>MGHHHHHHHHHHMSKQQIGVVGMAVMGRNLALNIESRGYTVSVFNRSREKTEEVIAENPGKKLVPYYTVQEFVESLETPRRILLMVKAGAGTDSAIDSLKPYLDKGDIIIDGGNTFFQDTIRRNRELSAEGFNFIGTGVSGGEEGTLKGPSIMPGGQKEAYELVAPILKQIAAVAEDGEPCVTYIGADGAGHYVKMVHNGIEYGDMQLIAEAYALLKGGLALSNEELAQTFTEWNEGELSSYLIDITKDIFTKKDE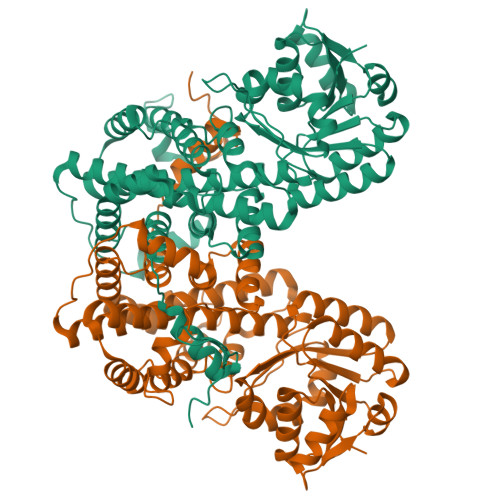EGKYLVDVILDEAANKGTGKWTSQSSLDLGEPLSLITESVFARYISSLKDQRVAASKVLSGPQAQPAGDKAEFIEKVRRALYLGKIVSYAQGFSQLRAASDEYNWDLNYGEIAKIFRAGCIIRAQFLQKITDAYAQNAGIANLLLAPYFKQIADDYQQALRDVVAYAVQNGIPVPTFSAAIAYYDSYRSAVLPANLIQAQRDYFGAHTYKRTDKEGIFHTEWLE[2x]> CCCGCGG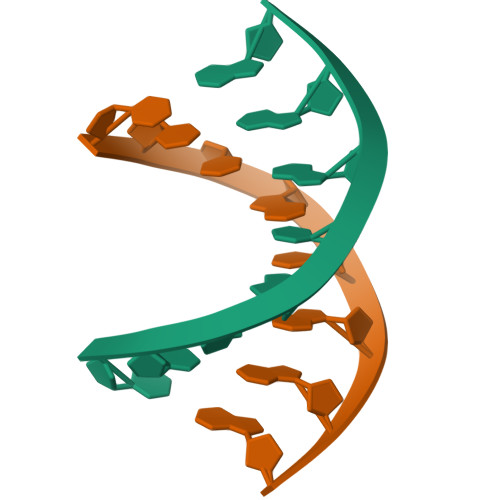G>[35x]MNHKVHHHHHHIEGRHMADKSTDLTVTEGGSDGALVASSDVDVESQNPDLEERSASKFDMAVGDLDLLRQVVLVLSISICVALIVMLFFWVKEPEMRPLGAYETEELIPVLDYLDQQKINYKLDGNTISVESSEYNSIKLGMVRSGVNQATEAGDDILLQDMGFGVSQRLEQERLKLSRERQLAQAIEEMKQVRKARVLLALPKHSVFVRHNQEASASVFLTLSTGTNLKQQEVDSIVDMVASAVPGMKTSRITVTDQHGRLLSSGSQDPASAARRKEQELERSQEQALREKIDSVLLPILGYGNYTAQVDIQMDFSAVEQTRKRFDPNTPATRSEYALEDYNNGNMVAGIPGALSNQPPADASIPQDVAQMKDGSVMGQGSVRKESTRNFELDTTISHERKQTGTVARQTVSVAIKDRRQVNPDTGEVTYTPMSESEINAIRQVLIGTVGFDQ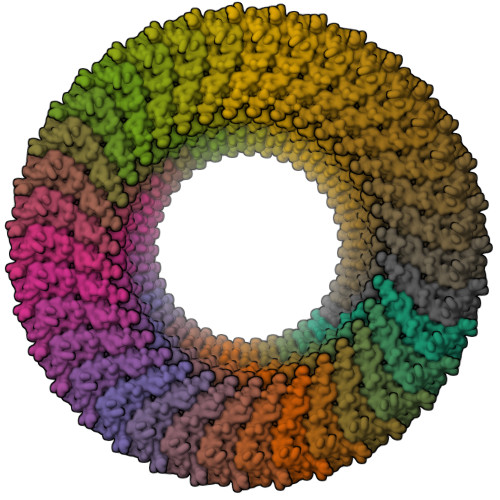GRGDLLNVLSVKFAEPEAEQLEEPPIWEHPNFSDWVRWFASALVIIVVVLVLVRPAMKKLLNPTSDDEDEMYGPDGLPIGADGETSLIGSDIESSELFEFGSSIDLPNLHKDEDVLKAVRALVANEPELAAQVVKNWMNDMANDIVPQDDNAAGMPVELDVSTITGEEKAAILLLSLNEQDAAGIIRHLEPKQVQRVGSAMAKAKDLSQDKVSAVHRAFLEDIQKYTNIGMGSEDFMRNALVAALGEDKANNLVDQILLGTGSKGLDSLKWMDPRQVASIIVNEHPQIQTIVLSYLEADQSAEILSQFPERVRLDLMMRIANLEEVQPSALAELNEIMEKQFAGQAGAQAAKISGLKAAAEIMNYLDNNVEGLLMEQIRDQDEDMATQIQDLMFVFENLVEVDDQGIQKLLRDVPQDVLQKALKGADDSLREKVFKNMSKRAAEMMRDDIEAMPPVRVADVEAAQKEILAIARRMADAGELMLSGGADEFL The cysteine protease legumain can develop asparaginyl endopeptidase (AEP) and carboxypeptidase (ACP) activities in a pH- and context-dependent manner. Primarily found in endolysosomes, legumain is involved in immunological processes such as antigen processing and TLR maturation as well as in tumor progression.

The crystal structure of hCE revealed the typical five-stranded antiparallel β-sheet wrapped around a central α-helix. Two disulfide bridges additionally stabilize the structure by clamping strands β4 and β5 and the hCE-specific appending structure that is inserted between strands β3 and β4. Parts of the appendix structure (Thr76–His82) were flexible in the electron density map. The legumain reactive center loop (RCL) of hCE exposed Asn39I in a conformation similar to that seen in hCC and hCF, consistent with its suggested role for active site (P1–S1) interaction.[4a] The conserved conformation of the RCL suggests a canonical, substrate-like binding mode that is shared within the type 2 cystatin family; differences in binding affinity within hCC/E/F should be related to exosite interactions. We considered Cys73I–Cys83I as one candidate for a legumain exosite loop (LEL) because it was stabilized relative to the reactive center loop (RCL) via charged interactions mediated by Lys75I to the P2 (Ser38I) and P1′ (Ser40I) carbonyls of the RCL.

> MDRPQERMVGELRDLSPDDPQVQKAAQAAVASYNMGSNSIYYFRDTHIIKAQSQLVAGIKYFLTMEMGSTDCRKTRVTGDHVDLTTCPLAAGAQQEKLRCDFEVLVVPWQNSSQLLKHNCVQMLEHHHHHH> MAEKEEAIFRSAEMALVQFYIPQEISRDSAYTLGQLGLVQFRDLNSKVRAFQRTFVNEIRRLDNVERQYRYFYSLLKKHDIKLYEGDTDKYLDGSGELYVPPSGSVIDDYVRNASYLEERLIQMEDATDQIEVQKNDLEQYRFILQSGDEFFLKGDNTDSTSYMDEDMIDANGENIAAAIGASVNYVTGVIARDKVATLEQILWRVLRGNLFFKTVEIEQPVYDVKTREYKHKNAFIVFSHGDLIIKRIRKIAESLDANLYDVDSSNEGRSQQLAKVNKNLSDLYTVLKTTSTTLESELYAIAKELDSWFQDVTREKAIFEILNKSNYDTNRKILIAEGWIPRDELATLQARLGEMIARLGIDVPSIIQVLD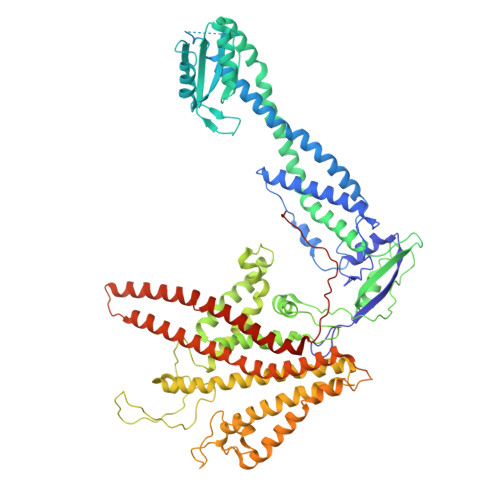TNHTPPTFHRTNKFTAGFQSICDCYGIAQYREINAGLPTIVTFPFMFAIMFGDMGHGFLMTLAALSLVLNEKKINKMKRGEIFDMAFTGRYIILLMGVFSMYTGFLYNDIFSKTMTIFKSGWKWPDHWKKGESITATSVGTYPIGLDWAWHGTENALLFSNSYKMKLSILMGFIHMTYSYFFSLANHLYFNSMIDIIGNFIPGLLFMQGIFGYLSVCIVYKWAVDWVKDGKPAPGLLNMLINMFLSPGTIDDELYPHQAKVQVFLLLMALVCIPWLLLVKPLHFKFTHKKKSHEPLPSTEADASSEDLEAQQLISAMDADDAEEEEVGSGSHGEDFGDIMIHQVIHTIEFCLNCVSHTASYLRLWALSLAHAQLSSVLWTMTIQIAFGFRGFVGVFMTVALFAMWFALTCAVLVLMEGTSAMLHSLRLHWVESMSKFFVGEGLPYEPFAFEYKDMEVAVASASSSASS> QYAPQTQSGRTSIVHLFEWRWVDIALECERYLGPKGFGGVQVSPPNENVVVTNPSRPWWERYQPVSYKLCTRSGNENEFRDMVTRCNNVGVRIYVDAVINHMCGSGAAAGTGTTCGSYCNPGSREFPAVPYSAWDFNDGKCKTASGGIESYNDPYQVRDCQLVGLLDLALEKDYVRSMIADYLNKLIDIGVAGFRIDASKHMW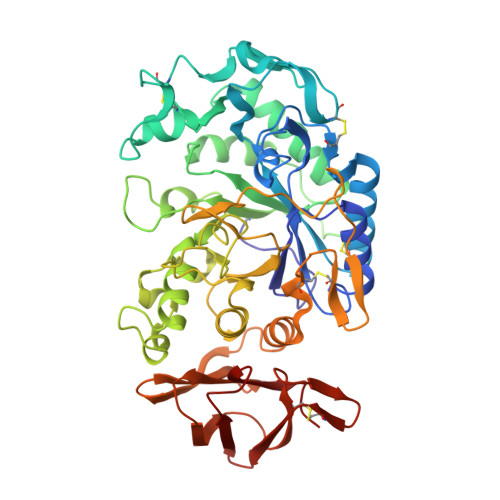PGDIKAVLDKLHNLNTNWFPAGSRPFIFQEVIDLGGEAIQSSEYFGNGRVTEFKYGAKLGTVVRKWSGEKMSYLKNWGEGWGFMPSDRALVFVDNHDNQRGHGAGGASILTFWDARLYKVAVGFMLAHPYGFTRVMSSYRWARNFVNGEDVNDWIGPPNNNGVIKEVTINADTTCGNDWVCEHRWREIRNMVWFRNVVDGQPFANWWDNGSNQVAFGRGNRGFIVFNNDDWQLSSTLQTGLPGGTYCDVISGDKVGNSCTGIKVYVSSDGTAQFSISNSAEDPFIAIHAESKL>[4x]AFVVTDNCIKCKYTDCVEVCPVDCFYEGPNFLVIHPD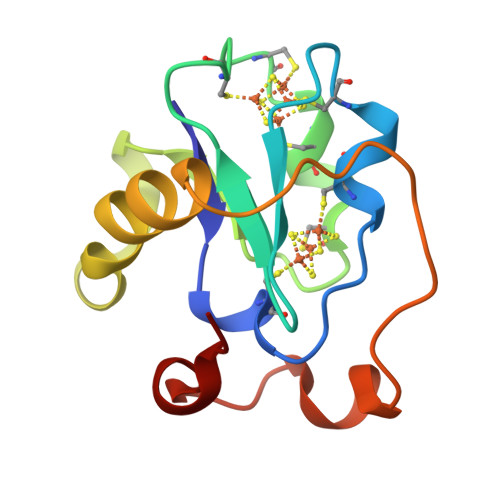ECIDCASCEPECPAQAIFSEDEVPEDMQEFIQLNAELAEVWPNITEKKDPLPDAEDWDGVKGKLQHLER The viral nucleoprotein (NP), a key component of the replication machinery, packages the viral genome into protective ribonucleoprotein particles. Although TiLV-NP is considerably smaller than its influenza counterpart and unrelated in sequence, it maintains the same topology and domain organisation. This comprises a head and body domain between which is a positively charged groove, where single-stranded RNA binds. In addition, an oligomerisation loop inserts into a hydrophobic pocket in the neighbouring NP, the flexible hinges of which allow variable orientation of adjacent NPs.

For the pseudo-C4 tetramer, the observed RNA is mostly single stranded, with one less well-ordered, double-stranded region. The pseudo-C2 and pseudo-C5 oligomers appeared the most stable with uniform density according to local resolution, while the pseudo-C4 and pseudo-C6 structures displayed poorer density for 2 and 3 NPs, respectively. To account for this variability, symmetry expansion, particle subtraction, 3D classification without alignments, and local refinements were applied during cryo-EM image processing (see ‘Materials and methods’). This enabled isolation and refinement of the most homogeneous sub-oligomers, corresponding to two NPs within each oligomer. Finally, 3D classification without alignments were performed to isolate the most homogeneous subset of particles, itself subjected to a final local refinement, resulting in four final maps enclosing 2 TiLV-NPs for each RNA-bound TiLV-NP oligomers (pseudo-C2/-C4/-C5/-C6).

>[3x]MVRTTKTSMAAASTVAPEVAMDEGSPSTSQAQVELPRNLEVFNEACGHVFGSSFNREDNSVISDAAAFLFKMHTHSLDGQEAKVLRASEKKRERENAKKSRKAPEAGMRVGRSLILTSRWTEYCATCVPALGSKMKVIKASGDAAMIQMMKDHNSLLRVCVRIEVWKARYVSLVALDERIQTLEDAQWFPYLSGDSYRACPGLVGGYFAKKAAAGERGKNYKKLNQTAIIPPPRFLIIGHRLQIGDQVTLRELLASIAWGLCDGVLAECWSPSQGDGSIGVVVGLPLQATGSCFLVVASHGLSAIADSRIEGTGNTNLLEECIAIQKQDGVIKCKRSGKSLYHCLKETAGAVGR>MAHHHHHHSSGLEVLFQGPNNTIINSLIGGDDSIKRSNVFAVDSQIPTLYMPQYISLSGVMTNDGPDNQAIASFEIRDQYITALNHLVLSLELPEVKGMGRFGYVPYVGYKCINHVSISSCNGVIWEIEGEELYNNCINNTIALKHSGYSSELNDISIGLTPNDTIKEPSTVYVYIKTPFDVEDTFSSLKLSDSKITVTVTFNPVSDIVIRDSSFDFETFNKEFVYVPELSFIGYMVKNVQIKPSFIEKPRRVIGQINQPTATVTEVHAATSLSVYTKPYYGNTDNKFISYPGYSQDEKDYIDAYVSRLLDDLVIVSDGPPTGYPESAEIVEVPEDGIVSIQDADVYVKIDNVPDNMSVYLHTNLLMFGTRKNSFIYNISKKFSAITGTYSDATKRTIFAHISHSINIIDTSIPVSLWTSQRNVYNGDNRSAESKAKDLFINDPFIKGIDFKNKTDIISRLEVRFGNDVLYSENGPISRIYNELLTKSNNGTRTLTFNFTPKIFFRPTTITANVSRGKDKLSVRVVYSTMDVNHPIYYVQKQLVVVCNDLYKVSYDQGVSITKIMGDNN[3x]

Trimeric capsomers of the VACV D13 protein form a transitory, stabilizing lattice on the surface of the initial spherical immature virus particle. The crystal structure of D13 reveals that this major scaffolding protein comprises a double β barrel “jelly-roll” subunit arranged as pseudo-hexagonal trimers. The D13 lattice seems to act as a mechanical scaffold for the growing crescent membrane of the IV with sufficient rigidity to maintain a constant radius of curvature of the crescents even before they close to form complete spheres (Chlanda et al., 2009; Heuser, 2005), thereby fixing the size of the immature virion.

The structure of native wild-type D13 was solved from the phases provided by the isomorphous SAD structure of D13D513G, and refined to 2.8 Å with R/Rfree = 0.177/0.206. Crystals for native and SeMet forms of both proteins were isomorphous and belonged to space group P6122, with one trimer in the crystallographic asymmetric unit. In both structures, continuous electron density is present from residues Ser15 to Met547; the final four residues (548–551) being disordered. The N-terminal hexahistidine tag is disordered in both structures. V1 and V2 jelly-rolls alternate around the molecular 3-fold axis, lending a pseudo-hexagonal symmetry to the lower part of the trimer. In contrast the three turret domains interact to form a cage that gives a triangular shape to the top of the trimer. The trimerization interface is completed by the N-terminal tail of each subunit (residues 15–31) that extends 43 Å from the V1 jelly-roll and wraps underneath the neighboring subunits locking the base of the trimer together. The triangular cage formed by the turret domains presents a negatively charged outer surface at the top of the trimer, whereas the N-terminal subunit tails form a positively charged surface at the base of the trimer close to the negatively charged membrane. D13D513G and wild-type D13 trimers differ only in the additional short N-terminal helix (residues 2–10) visualized in the structure of D13D513G.> EILDLTQTLINFPRPGDPELRIIEKKIDGFIVSEIIMGSHLCTHIDYPKHVGLENRIPFKDGIIKGKGYCISLDDFPGNKLPACDILLIYTGFSKYWGRDEYFEKIPEIPFLDDIIKSNIKCVGIDACTIGGFEE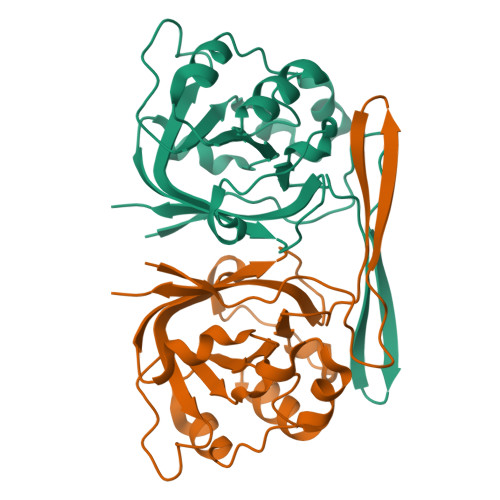HKRLLSNNILIIENLNENLKNLVGKSFYFLGLPLKIFDIDASPIRCIAILE> RQVIVPVCMPKIHYSPLKTGLCYDVRMRYHAKIFTSYFEYIDPHPE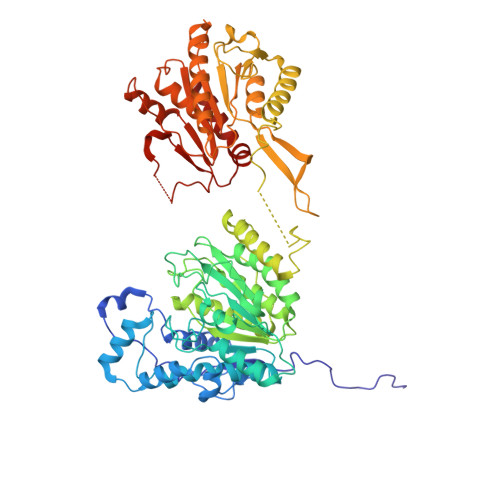DPRRIYRIYKILAENGLINDPTLSGVDDLGDLMLKIPVRAATSEEILEVHTKEHLEFIESTEKMSREELLKETEKGDSVYFNNDSYASARLPCGGAIEACKAVVEGRVKNSLAVVRPPGHHAEPQAAGGFCLFSNVAVAAKNILKNYPESVRRIMILDWDIHHGNGTQKSFYQDDQVLYVSLHRFEMGKYYPGTIQGQYDQTGEGKGEGFNCNITWPVGGVGDAEYMWAFEQVVMPMGREFKPDLVIISSGFDAADGDTIGQCHVTPSCYGHMTHMLKSLARGNLCVVLEGGYNLDAIARSALSVAKVLIGEPPDELPDPLSDPKPEVIEMIDKVIRLQSKYWNCFRRRHANSGCNFNEPINDSIISKNFPLQKAIRQQQQHYLSDEFNFVTLPLVSMDLPDNTVLCTPNISESNTIIIVVHDTSDIWAKRNVISGTIDLSSSVIIDNSLDFIKWGLDRKYGIIDVNIPLTLFEPDNYSGMITSQEVLIYLWDNYIKYFPSVAKIAFIGIGDSYSGIVHLLGHRDTRAVTKTVINFLGDKQLKPLVPLVDETLSEWYFKNSLIFSNNSHQCWKENESRKPRKKFGRVLRCDTDGLNNIIEERFEEATDFILDSFE> MISQSRYIRIISGVGAGAPVAGRKLILRVMTTNNVIPPGIVIEFDNSNAVMSYFGAQSEEYQRAAAYFKFISKSVNSPSSISFARWVNTAIAPMVVGDNLPKTIADFAGFSAGVLTIMVGAAEKNITAIDTSAATSMDNVASIIQTEIRKNTDPQLAQATVTWNQNTNQFTLVGATIGTGVLAVAKSADPQDMSTALGWSTSNVVNVAGQAADLPDAAVAKSTNVSNNFGSFLFAGAPLDNDQIKAVSAWNAAQNNQFIYTVATSLANLGTLFDLVKGNAGTGLHVLSATAANDFVEQCPSEIFAATNYDEPGASQNYMYYQFPGRNITVSDDTVANTVDKSRGNYIGVTQAN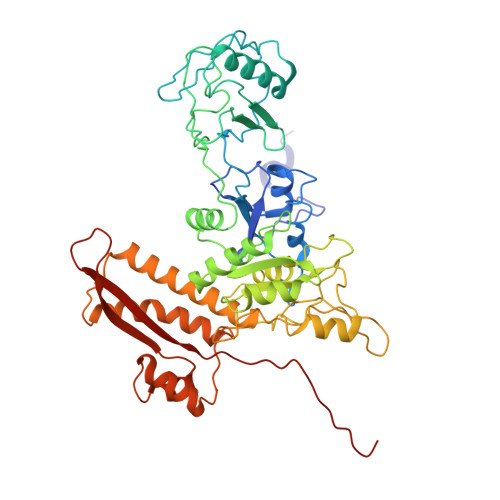GQQLAFYQRGILCGGPTDAVDMNVYANEIWLKSAIAQALLDLFLNVNAVPASSTGEAMVLAVLQPVLDKATANGTFTYGKEISAVQQQYITQVTGDRRAWRQVQTLGYWINITFSSYTNNNTGLIEWKANYTLIYSKGDAIRFVEGSDVMI> SNATDTAEQVIASFRILASDKPYILAEELRRELPPDQAQ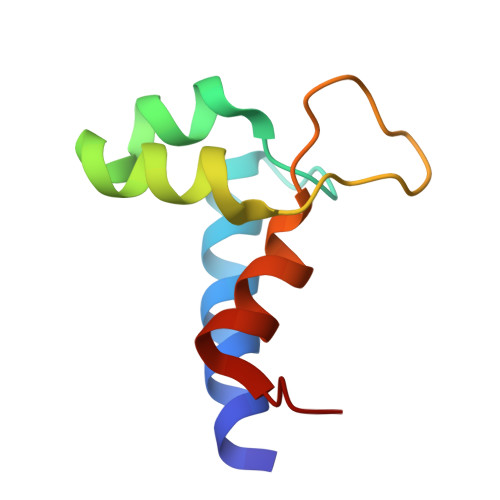YCIKRMPAYSGPGSVPGALDYAAFSSALYGESDL> MPDASLFNGTSFITLFAPNISLLQASIDFYTNFLGFAIRKNSNQKLFWLQLEEDQNNVSIQLILDPEHAASVSQIDQNIRNLTRSLYRKDWRSIQSNIAFKSSSLSKLVKLLKDGGHPVQQSPNEISPFEVYTVDPLGSLIGFSGFKNPFAVNERSLLPKVSEEKAYRAEDDSEKLLNPVRKTIGVMTSGGDSPGMNPFVRAVVRAGIYKGCKVFCIHEGYEGLVRGGEKYIKETQWHDVRGWLVEGGTNIGTARCKEFRERSGRLKACKNMIDMGIDALIVCGGDGSLTGADRFRSEWPSLIEELLQTEQISQQQFNTHQNLNICGAVGSIDNDMSSTDATIGAFSSLDRICRAIDYIDATANSHSRAFIVEVMGRHCGWLGLLAGLATSADYILIPEKPASSREWQDQMCDIVGKHRARGKRKTIVIVAEGAISNDLSPISCDQVKDVLVNRLGLDTRVTTLGHVQRGGTAVAFDRIYATLQGVEAVNAVLECDADTPSPMIAIKEDQITRVPLVDAVELTQQVAKSIESRNFKKAISLRDSEFVEHMKNFISTN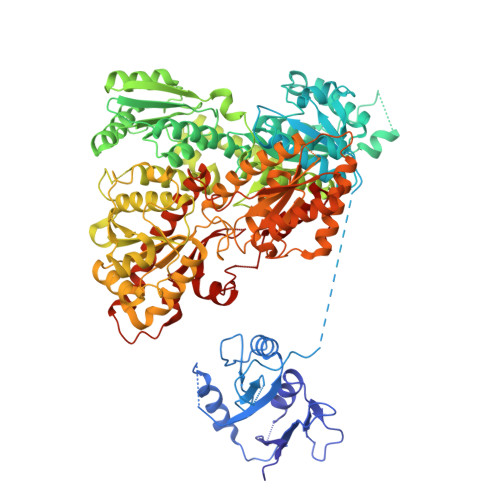SADHVPPSLPLEKRKKIAIINVGAPAGGMNSAVYSMATYCMSRGHVPYAIHNGFSGLARHESVRSINWLDIEGWGSLGGSEIGTNRTLPNDADIGMIAYFFEKYGFDGLILVGGFEAFISLHQLERARINYPSLRIPLVLIPATISNNVPGTEYSLGSDTCLNSFMEYCDVIKQSAAATRNRVFVVEVQGGNSGYIATHAQLACGAQISYVPEEGISLAQLEMDINSLKESFANDQGKTKSGRLILKSENASKVLTTEVISTIIDDEASGRFDSKTAIPGHVQQGGIPSPMDRVRASRFAIRAVSFIERHSDRCQTFKNSISFRQTDEITSTAVVLGIHKSQLRFTPIRQLYDFESDVPRRMRKNIFWSNVREISDMLSGRTSL> GSSMGSLNQDATILRQAKLGLSDPAQSLSSWSDNNDVTPCKWLGVSCDATSNVVSVDLSSFMLVGPFPSILCHLPSLHSLSLYNNSINGSLSADDFDTCHNLISLDLSENLLVGSIPKSLPFNLPNLKFLEISGNNLSDTIPSSFGEFRKLESLNLAGNFLSGTIPASLGNVTTLKELKLAYNLFSPSQIPSQLGNLTELQVLWLAGCNLVGPIPPSLSRLTSLVNLDLTFNQLTGSIPSWITQLKTVEQIELFNNSFSGELPESMGNMTTLKRFDASMNKLTGKIPDNLNLLNLESLNLFENMLEGPLPESITRSKTLSELKLFNNRLTGVLPSQLGANSPLQYVDLSYNRFSGEIPANVCGEGKLEYLILIDNSFSGEISNNLGKCKSLTRVRLSNNKLSGQIPHGFWGLPRLSLLELSDNSFTGSIPKTIIGAKNLSNLRISKNRFSGSIPNEIGSLNGIIEISGAENDFSGEIPESLVKLKQLSRLDLSKNQLSGEIPRELRGWKNLNELNLANNHLSGEIPKEVGILPVLNYLDLSSNQFSGEIPLELQNLKLNVLNLSYNHLSGKIPPLYANKIYAHDFIGNPGLCVDLDGLCRKITRSKLEGSENLYFQ;> YPKGVPIPPSAPSKRHN

The LRR-RKs HAESA (greek: to adhere to) and HAESA-LIKE 2 (HSL2) redundantly control floral abscission. A receptor protein called HAESA is found on the surface of the cells that surround a future break point on the plant. When its time to shed an organ, a hormone called IDA instructs HAESA to trigger the shedding process. The peptide hormone IDA binds to the HAESA LRR ectodomain.

We next investigated whether HAESA binds N-terminally extended versions of IDA. We obtained a structure of HAESA in complex with a PKGV-IDA peptide at 1.94 Å resolution. In this structure, no additional electron density accounts for the PKGV motif at the IDA N-terminus. Consistently, PKGV-IDA and IDA have similar binding affinities in our ITC assays, further indicating that HAESA senses a dodecamer peptide comprising residues 58-69IDA. The PKGV motif present in our N-terminally extended IDA peptide is highlighted in red. While the sequence of the mature IDA peptide has not been experimentally determined in planta, our HAESA-IDA complex structures and calorimetry assays suggest that active IDLs are hydroxyprolinated dodecamers.> SGRPMDKCWFTLDNAHYPPPSLDSMRSGHPISPASLGHLIPSLAHLDQIINAKAIEPFPATMDIHGPTIIED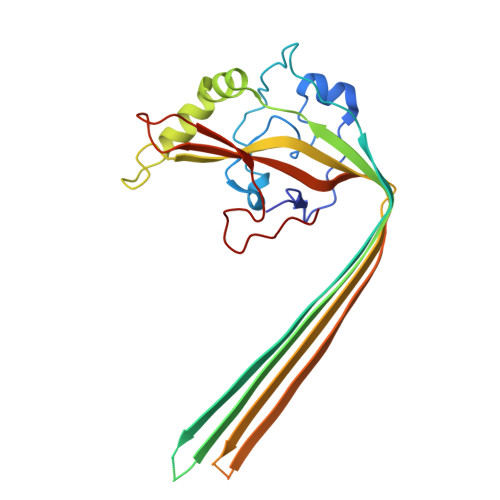FKWDHSHEYSLSLGGKVPIPLAPAGVPFVDLNVGLGGAFSRSVANYWEFDRLERYIMQPTRSYVQKCIERDEVKRWIAKNKSMMMMGRWEVYMITGIIVARGGGRKKKEKTTGKEFSVEVTVEVPLIVEAGPGGKRNTARQKTWGTSQTGDFVWAVRLAKITKSGLHSDWKMETVFGKTSSFRGQKAIF>[4x]GMKMLEQLEKKLGYTFKDKSLLEKALTHVSYSKKEHYETLEFLGDALVNFFIVDLLVQYSPNKREGFLSPLKAYLISEEFFNLLAQKLELHKFIRIKRGKINETIIGDVFEALWAAVY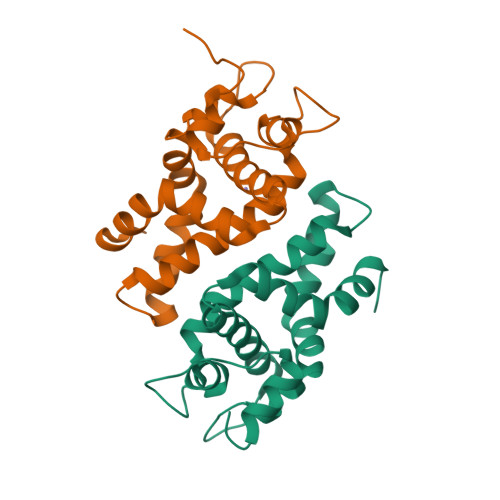IDSGRDANFTRELFYKLFKEDILSAIKEGRHHHHHH>[4x]ADTTTAAPADAKPMMHHKGKFGPHQDMMFKDLNLTDAQKQQIREIMKGQRDQMKRP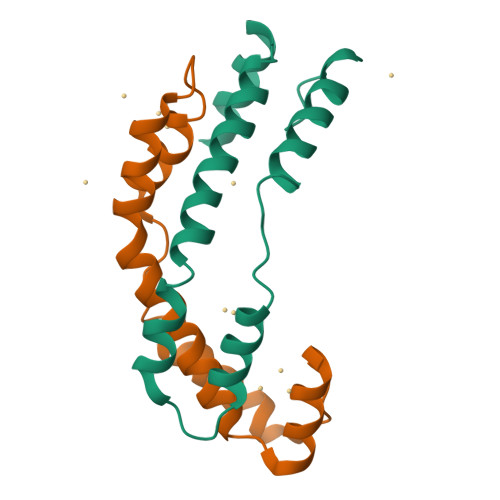PLEERRAMHDIITSDTFDKVKAEAQIAKMEEQRKANMLAHMETQNKIYNILTPEQKKQFNANFEKRLTERPAAKGKMPATAE> MIKIIKNAKVFSPEYIGKKDVIFYHKVIHVGEGVNTSVLPFEHEIYDANGLLLLPGLIDPHVHITGGGGEGGFETRTPELKISDCIRSGVTTVVGCLGTDGITRSLENLYAKAKSLESEGLNTFIYTGSYRVPPVTFTGSIMRDIVLIDKVIGVGEIAISDHRSSQPTLEEILRIVADIRVGGMISGKAGIVNFHVGSGKRGIEYLFDIIEKTEIPIQHLYPTHMSRSRKLFEQGLEFAKRGGTIDLTALQPKDAEFVRAEFTTIDAICEAYENGLLDNVTISSDGQGSLPKFDDNGNFVGLDVGSVSAVWYTIRKVLEKGLPLAEVLKISTTNPARVFKLNKGKIAKGQDADFILVDEQSFEIVSVISKGEFLMKDGVMKNLNFEF

In the present study, we functionally characterized the hyperthermophilic M38 β-aspartyl peptidase FiBAP, a protein repair enzyme involved in hydrolysis of isoAsp residue-containing peptides in F. islandicum AW-1. The overall structure of each monomer can be divided into two distinct domains; an N-terminal β-sandwich domain (M1–G56; G344–E386) and a C-terminal catalytic domain (L57–K343), that are mainly involved in dimerization and catalysis, respectively. The catalytic domain at the C-terminus of the molecule folds into a (β/α)8 triosephosphate isomerase (TIM)-barrel motif.

Crystal structures of the ligand-free form of FiBAP and the ligand-bound form bound with N-carbobenzoxy-β-Asp-Leu (Cbz-β-DL) as a substrate analog were determined at resolutions of 2.6 and 2.7 Å, respectively. Cbz-β-DL-free and -bound structures belonged to I422 and P2212 space groups, with one and four subunits in the asymmetric unit, respectively. The ligand-free model included most amino acids except for residues D254–R259 and P290–L302, corresponding to the flexible loops in the molecule. Zn1 is coordinated by E156, H195, and H224 residues, while Zn2 is bound by H61, H63, E156, and D285. In the metal coordination network, Zn1 interacts with Zn2 via E156. In addition, E156 in FiBAP forms a cis-peptide bond with G155 in the loop between α4 and β10, which is conserved in the corresponding loop of CpIadA between G165 and E166. The cis-peptide bond favors loop bending in FiBAP, which positions E156 toward the metal, as opposed to the carbamylated lysine (KCX162) in EcIadA, suggesting that FiBAP belongs to the Type-I IadAs. Similar to EcIadA and CpIadA, size-exclusion chromatography indicated that FiBAP is an octamer in solution, usually referred to as a “tetramer of dimers”, as supported by symmetry-related molecule analysis. The initial dimer is formed when the β-sandwich domain of each monomer interacts with an adjacent monomer, mainly through hydrophobic interactions involving several residues (I2, I4, V34, V35, V38, L39, F41, and I46) in the loop between β4 and β5. Additionally, the substrate-binding cavity of the catalytic domain participates in dimerization by providing the second point of contact between adjacent partners through salt bridges. These four salt bridges are formed by E107 (α2), K114 (α2), R143 (α3), and D149 (α3) of each monomer of the dimer.>[4x]QTNVELKTPAQKASYGIGLNMGKSLSQEGMDDLDSKAVAKGIEDALGKKKQQLTD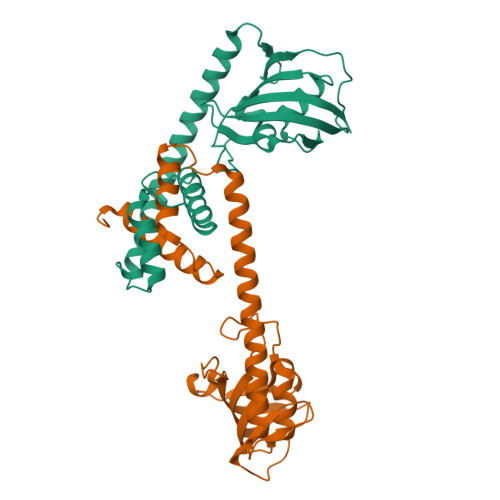EELTEAFAFLQKRAEERMAAIGDENAKAGKKFLEENGKRDGVTTTASGLQYEIVKKADGPQPKATDVVTVHYEGRLTDGTVFDSSIERGSPIDLPVSGVIPGWVEALQLMHVGEKIKLYIPSELAYGAQSPSPAIPANSVLVFDMELLGIKDP> GPLGSPEFMIWERLIKWKDETIEVLNNNLVEYNEPGMERFNNEKLGWVNRTWNNRYIRRAHLDVVDVRESKGLWMAHLCLFPMLTNGGPIYGFDIIAGEKKVTGAFHDFSPLLQKDHPLTKWFIEENKWFKPSKERELPEWAKAIFSGGM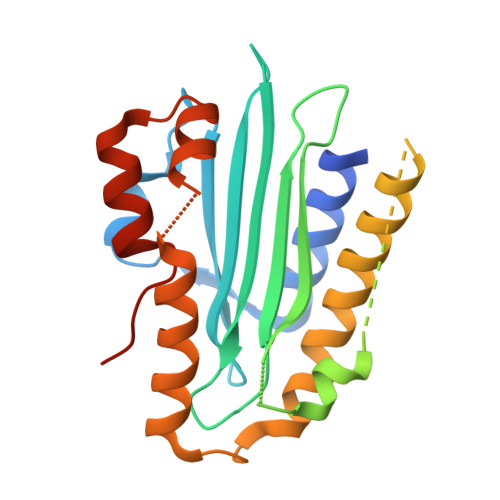IAAGNVREEDELNKICTMAVSNLNNYIDKIRNHEGEAEMADVIKAQNYYSEHQQKNPHTPRVMQSLGLPEEDIKLFCSDNLFPFVSENQPYLK>[8x]SMEYGHHARPDSKRPLDEGSPAAAGLTSKKANEALTRNRELTTVLVKNL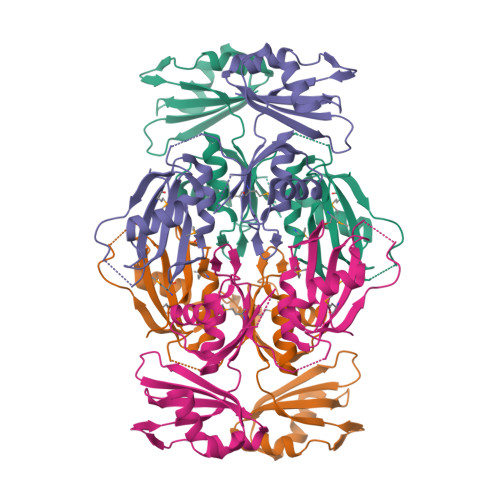PKSYNQNKVYKYFKHCGPIIHVDVADSLKKNFRFARIEFARYDGALAAITKTHKVVGQNEIIVSHLTECTLWMTNFPPSYTQRNIRDLLQDINVVALSIRLPSLRFNTSRRFAYIDVTSKEDARYCVEKLNGLKIEGYTLVTKVSNPLEKSKRTDSATLEGREIMIRNLSTELLDENLLRESFEGFGSIEKINIPAGQKEHSFNNCCAFMVFENKDSAERALQMNRSLLGNREISVSLADKKP>MHHHHHHADLAESNIKVMCRFRPLNESEVNRGDKYIAKFQGEDTVVIASKPYAFDRVFQSSTSQEQVYNDAAKKIVKDVLEGYNGTIFAYGQTSSGKTHTMEGKLHDPEGMGIIPRIVQDIFNYIYSMDENLEFHIKVSYFEIYLDKIRDLLDVSKTNLSVHEDKNRVPYVKGATERFVSSPDEVMDTIDEGKSNRHVAVTNMNEHSSRSHSIFLINVKQENTQTEQKLSGKLYLVDLAVSEKVSKTGAEGAVLDEAKNINKSLSALGN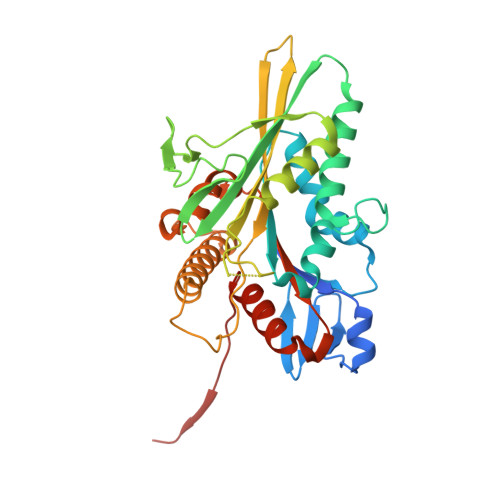VISALAEGSTYVPYRDSKMTRILQDSLGGNARTTIVICCSPSSYNESETKSTLLFGQRAKTIKNTVSVNVELT[2x]Rspo (R-spondin, also roof plate-specific spondin) proteins are evolutionarily conserved from fish to humans and have well-documented roles in a broad range of developmental and physiological processes resulting from enhancement of canonical and non-canonical Wnt signalling. ZNRF3/RNF43 specifically targets these Wnt receptors for ubiquitination and turnover, hence reducing Wnt signalling responses. Direct extracellular interaction with Rspo proteins inhibits ZNRF3/RNF43 activity. Here we report a molecular level analysis of the ZNRF3/RNF43 ectodomain structure and its interactions with Rspo proteins.

The ZNRF3ecto crystal structures revealed a distinctive variant of the protease-associated domain topology. Two β-sheets (comprising β2, β1, β7, β3 and β4, β5, β6 strands, respectively) splay apart, accommodating an α-helix (αC) at the open edge; two additional α-helices (αA and αB) pack against the β4, β5 and β6 face of this distorted β-sandwich. A disulphide bridge, conserved across species, links two structurally elaborate loops, β3–β4 and β4–αA. The crystal structures for apo xZNRF3ecto, zZNRF3ecto and mZNRF3ecto showed no major differences in the main chain conformation. Comparisons of ZNRF3ecto structures for proteins crystallized in several different crystal lattices, or for crystals containing multiple copies in the asymmetric unit, consistently highlighted an acidic region (N105-E114; residue numbering is for mouse sequences unless otherwise stated) within the β3–β4 loop, the short αC–β7 loop and the extended β1–β2 hairpin as flexible elements of the fold. Our crystallographic data provided independent structures for multiple copies of the ZNRF3 ectodomain in eight different crystal forms. All but two of these crystal structures reveal an extensive interface (average interface area 992±109 Å2) formed between two ZNRF3ecto polypeptide chains. This dimer is conserved, and pairwise structural superpositions yielded r.m.s.d. values of <1.3 Å (for 275 equivalent Cα pairs). The interaction is twofold symmetric; strands β3 and β7 of the ‘subunits’ abut face-to-face at the core of the dimer. The β1–β2 hairpin forms a second interface by reaching out to embrace helix αA and the β3–β4 loop in the opposing subunit.

>[3x]ETGKETAFVEVVLFESSPSGDYTTHTTGLTGRFSRAGAMLSAEGEIVQMHPLGLCNNNDEEDLYEYGWVGVVKLEQPELDPKPCLTVLGKAKRAVQRGATAVIFDVSENPEAIDQLNQGSEDPLKRPVVYVKGADAIKLMNIVNKQKVARARIQHLGTKHHHHHH> VGLTTLFWLGAIGMLVGTLAFAWAGRDAGSGERRYYV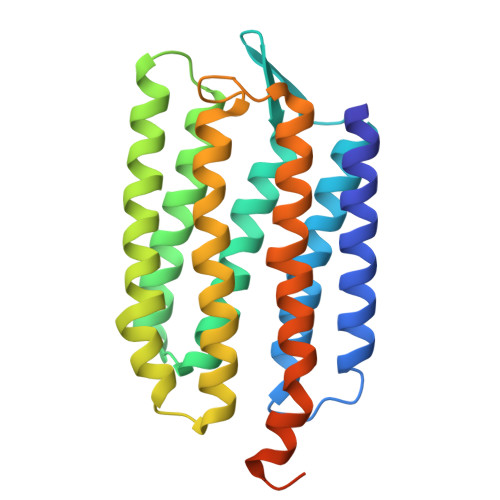TLVGISGIAAVAYVVMALGVGWVPVAERTVFAPRYIDWILTTPLIVYFLGLLAGLDSREFGIVITLNTVVMLAGFAGAMVPGIERYALFGMGAVAFLGLVYYLVGPMTESASQRSSGIKSLYVRLRNLTVILWAIYPFIWLLGPPGVALLTPTVDVALIVYLDLVTKVGFGFIALDAAATLRAEHGESLAGVDTDAPAVADENSHHHHHHH> CGRFAQSQTREDYLALLAEDIERDIPYDPEPIGRYNVAPGTKVLLLSERDEHLHLDPVFWGYAPGWWDKPPLINARVETAATSRMFKPLWQHGRAICFADGWFEWKKEGDKKQPFFIYRADGQPIFMAAIGSTPFERGDEAEGFLIVTAAADQGLVDIHDRRPLVLSPEAAREWMRQEISGKEASEIAASGCVPANQ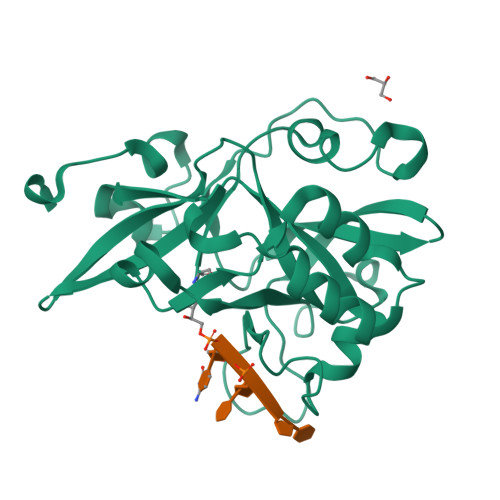FSWHPVSRAVGNVKNQGAELIQPVLEVLFQ>VTSSPFKTIKSDEIFAAAQKLMPGGVSSPVRAFKSVGGQPIVFDRVKDAYAWDVDGNRYIDYVGTWGPAICGHAHPEVIEALKVAMEKGTSFGAPCALENVLAEMVNDAVPSIEMVRFVNSGTEACMAVLRLMRAYTGRDKIIKFEGCYHGHADMFLVKAGSGVATLGLPSSPGVPKKTTANTLTTPYNDLEAVKALFAENPGEIAGVILEPIVGNSGFIVPDAGFLEGLREITLEHDALLVFDEVMTGFRIAYGGVQEKFGVTPDLTTLGKIIGGGLPVGAYGGK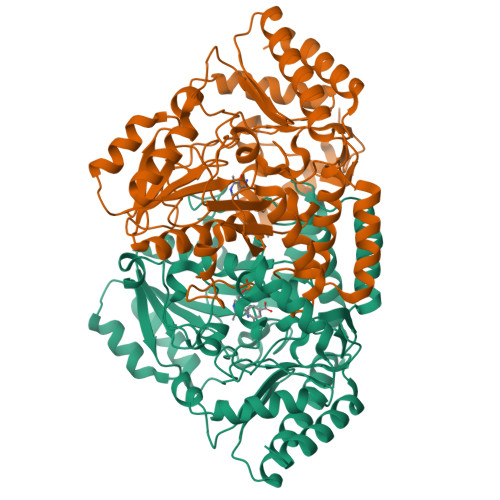REIMQLVAPAGPMYQAGTLSGNPLAMTAGIKTLELLRQPGTYEYLDQITKRLSDGLLAIAQETGHAACGGQVSGMFGFFFTEGPVHNYEDAKKSDLQKFSRFHRGMLEQGIYLAPSQFEAGFTSLAHTEEDIDATLAAARTVMSAL[2x]>[2x]ADTI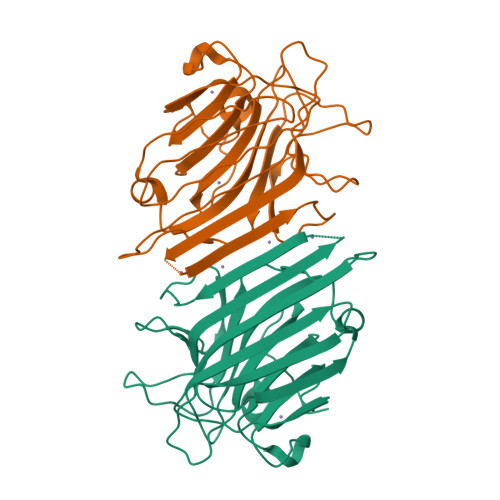VAVELDSYPNTDIGDPSYPHIGIDIKSIRSKSTARWNMQTGKVGTAHISYNSVAKRLSAVVSYTGSSSTTVSYDVDLNNVLPEWVRVGLSATTGLYKETNTILSWSFTSKLKTNSIADANSLHFSFNQFSQNPKDLILQGDATTDSDGNLELTKVSSSGDPQGSSVGRALFYAPVHIWEKSAVVASFDATFTFLIKSPDRDPADGITFFIANTDTSIPSGSGGRLLGLFPDAN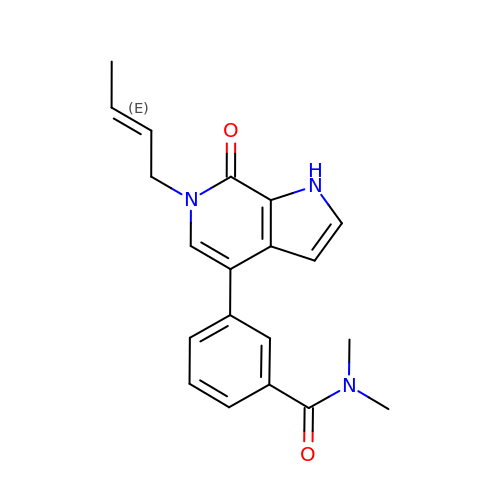3-{6-[(2E)-but-2-en-1-yl]-7-oxo-6,7-dihydro-1H-pyrrolo[2,3-c]pyridin-4-yl}-N,N-dimethylbenzamide | C20 H21 N3 O2 | RJEMCUZKQLRUIS-SNAWJCMRSA-N> VVRVADTMPSGPSNSESIPALTAAETGHTSQVVPSDTIQTRHVRNFHVRSESSVENFLSRSACVYIVEYKTR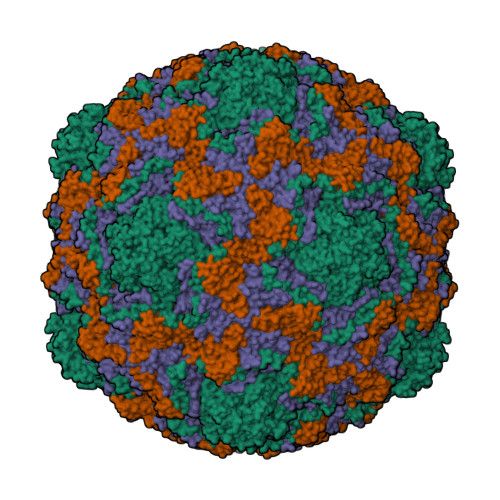DDTPDKMYDSWVINTRQVAQLRRKLEFFTYVRFDVEVTFVITSVQDDSTRQNTDTPALTHQIMYVPPGGPIPQAVDDYNWQTSTNPSVFWTEGNAPPRMSIPFMSVGNAYSNFYDGWSHFSQTGVYGFNTLNNMGKLYFRHVNDKTISPITSKVRIYFKPKHVKAWVPRPPRLCEYTHKDNVDFEPKGVTTSRTQLTISNSTH;> SDRVRSITLGNSTITTQESANVVVGYGVWPDYLSDEEATAEDQPTQPDVATCRFYTLDSVSWMKESQGWWWKFPDALRDMGLFGQNMQYHYLGRSGYTIHVQCNASKFHQGCLLVVCVPEAEMGAANINEKINREHLSNGEVANTFSGTKSSNTNDVQQAVFNAGMGVAVGNLTIFPHQWINLRTNNCATIVMPYINSVPMDNMFRHYNFTLMIIPFAKLDYAAGSSTYIPITVTVAPMCAEYNGLRLAGHQ;> GLPVMNTPGSNQFLTSDDYQSPTAMPQFDVTPEMNIPGEVKNLMEIAEVDSVVPVNNVNENVNSLEAYRIPVHSVTETGAQVFGFTLQPGADTVMERTLLGEILNYYANWSGSIKLTFMYCGSAMATGKFLLAYSPPGAGVPKNRREAMLGTHIIWDIGLQSSCVLCVPWISQTHYRFVSKDIYTDAGFITCWYQTSIVVPAEVQNQSVILCFVSACNDFSVRLLRDSPFVRQTAFYQ;> GAQVSTQKTGAHETSLSASGNSIHYTNINYYKDAASNSANRQDFTQDPGKFTEPVKDIMVKSLPALN>MVTVGNYCEAEGPVGPAWMQDGLSPCFFFTLVPSTRMALGTLALVLALPCRRRERPAGADSLSWGAGPRISPYVLQLLLATLQAALPLAGLAGRVGTARGAPLPSYLLLASVLESLAGACGLWLLVVERSQARQRLAMGIWIKFRHSPGLLLLWTVAFAAENLALVSWNSPQWWWARADLGQQVQFSLWVLRYVVSGGLFVLGLWAPGLRPQSYTLQVHEEDQDVERSQVRSAAQQSTWRDFGRKLRLLSGYLWPRGSPALQLVVLICLGLMGLERALNVLVPIFYRNIVNLLTEKAPWNSLAWTVTSYVFLKFLQGGGTGSTGFVSNLRTFLWIRVQQFTSRRVELLIFSHLHELSLRWHLGRRTGEVLRIADRGTSSVTGLLSYLVFNVIPTLADIIIGIIYFSMFFNAWFGLIVFLCMSLYLTLTIVVTEWRTKFRRAMNTQENATRARAVDSLLNFETVKYYNAESYEVERYREAIIKYQGLEWKSSASLVLLNQTQNLVIGLGLLAGSLLCAYFVTEQKLQVGDYVLFGTYIIQLYMPLNWFGTYYRMIQTNFIDMENMFDLLKEETEVKDLPGAGPLRFQKGRIEFENVHFSYADGRETLQDVSFTVMPGQTLALVGPSGAGKSTILRLLFRFYDISSGCIRIDGQDISQVTQASLRSHIGVVPQDTVLFNDTIADNIRYGRVTAGNDEVEAAAQAAGIHDAIMAFPEGYRTQVGERGLKLSGGEKQRVAIARTILKAPGIILLDEATSALDTSNERAIQASLAKVCANRTTIVVAHRLSTVVNADQILVIKDGCIVERGRHEALLSRGGVYADMWQLQQGQEETSEDTKPQTMERDYKDDDDK[2x]

One superfamily member, human ATP-binding cassette sub-family B member 6 (ABCB6), has been implicated in several seemingly disparate diseases. ABCB6 is expressed ubiquitously as a half transporter which homodimerizes to form a functional transporter. ABCB6 is a porphyrin transporter that is abundant in erythroid cells, where it is capable of accelerating porphyrin biosynthesis and protecting against porphyrin overload. ABCB6 has been implicated in dyschromatosis universalis hereditaria, a condition characterized by hyperpigmented and hypopigmented skin macules.

Several cryo-EM structures of ABCB6 have been reported, and here we report an additional high-resolution structure (2.93 Å) of human ABCB6. We purified ABCB6 in the presence of n-dodecyl-β-maltoside (DDM) / cholesteryl hemisuccinate (CHS) and obtained a reconstruction of ABCB6 to a resolution of 3.5 Å. Our final model is in good agreement with other deposited ABCB6 structures in the inward-facing conformation. Notably, the resolution of our cryo-EM structure (2.93 Å) is higher than previous cryo-EM structures. In addition to the canonical TMD and NBD, ABCB6 contains an additional N-terminal TMD termed TMD0. In most of the published structures in detergent and nanodiscs, including our own, density for the TMD0 is missing from the final model. In our preparation of ABCB6 in DDM/CHS, the TMD0 is too flexible to emerge in the 2D class projections. We prioritized the global resolution of the structure over the TMD0 so that the resulting structure would be appropriate for MD simulations. Using our cryo-EM structure of ABCB6 WT, MD simulations were employed to study the effect of the L356P mutation on ABCB6 structure. Conversely, the elongated loop of the L356P mutant extended across the ATP binding site, occluding the site, and causing direct clashes with the overlayed binding conformation of ATP.> GGCUUAUCAAGAGAGGGCGAGGGACUGGCCCGACGACCCCCGGCAACCAGAAAUGGUGCCAAUUCCUGCAGCGGAAACGUUG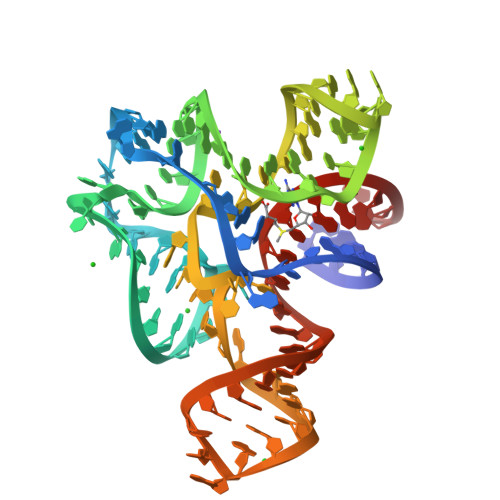AAAGAUGAGCCG N-glycolyl-alpha-neuraminic acid | C11 H19 N 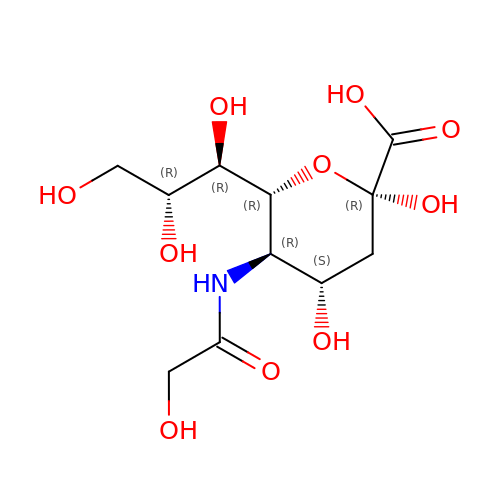O10 | FDJKUWYYUZCUJX-VTERZIIISA-N>MSLEQASVTNDFS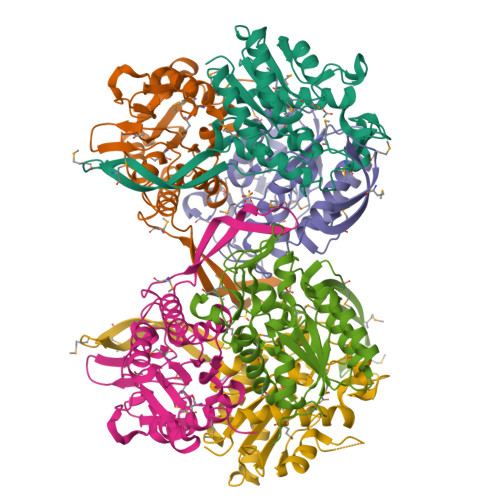ENKQGCIQHPWQGKKVGYIGDSITDPNCYGDNIKKYWDFLKEWLGITPFVYGISGRQWDDVPRQAEKLKKEHGGEVDAILVFMGTNDYNSSVPIGEWFTEQEEQVLSAHGEMKKMVTRKKRTPVMTQDTYRGRINIGITQLKKLFPDKQIVLLTPLHRSLANFGDKNVQPDESYQNGCGEYIDAYVQAIKEAGNIWGIPVIDFNAVTGMNPMVEEQLIYFYDAGYDRLHPDTKGQERMARTLMYQLLALPVAFEGHHHHHH[6x]> MSNDHLETTGSSDPNTNLLKYLPIVLNPDRTITRPIQIPSTAASPDPTSSSPVLTKDLALNPLHNTFVRLFLPRHALYNSAKLPLVVYFHGGGFILFSAASTIFHDFCCEMAVHAGVVIASVDYRLAPEHRLPAAYDDAMEALQWIKDSRDEWLTNFADFSNCFIMGESAGGNIAYHAGLRAAAVADELLPLKIKGLVLDEPGFGGSKRTGSELRLANDSRLPTFVLDLIWELSLPMGADRDHEYCNPTAESEPLYSFDKIRSLGWRVMVVGCHGDPMIDRQMELAERLEK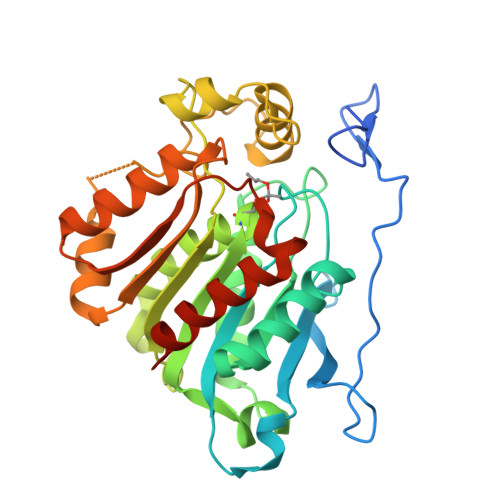KGVDVVAQFDVGGYHAVKLEDPEKAKQFFVILKKFVVDSCTTKLKLN>MEAVPRMPMIWLDLKEAGDFHFQPAVKKFVLKNYGENPEAYNEELKKLELLRQNAVRVPRDFEGCSVLRKYLGQLHYLQSRVPMGSGQEAAVPVTWTEIFSGKSVAHEDIKYEQACILYNLGALHSMLGAMDKRVSEEGMKVSCTHFQCAAGAFAYLREHFPQAYSVDMSRQILTLNVNLMLGQAQECLLEKSMLDNRKSFLVARISAQVVDYY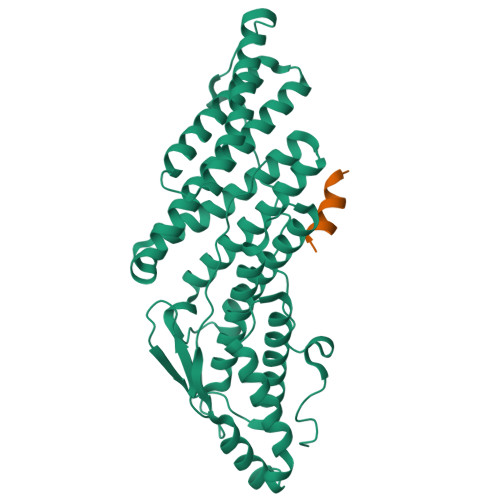KEACRALENPDTASLLGRIQKDWKKLVQMKIYYFAAVAHLHMGKQAEEQQKFGERVAYFQSALDKLNEAIKLAKGQPDTVQDALRFTMDVIGGKYNSAKKDNDFIYHEAVPALDTLQPVKGAPLVKPLPVNPTDPAVTGPDIFAKLV[4x];>[4x]PKVDEDEEALKQLAEWVS>[2x]SNAMTEKEKMLSGKGYYANDELLVKEREYCKKLTRLFNNTLEDEYEKREDILRQLFGSVGKQINVEQNIRCDYGYNIHVGENFFANYDCIFL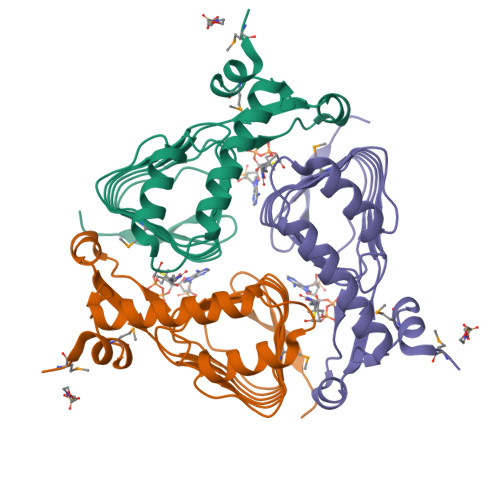DVCKIEIGDNVMLAPNVQIYTAYHPIDAQLRNSGIEYGSPVKIGDNVWIGGGVIITPGITIGDNVVIGAGSVVTKDIPPNTVAVGNPCRVIKKIEE> MTFTVDITPKTPTGVIDETKQFTATPSGQTGGGT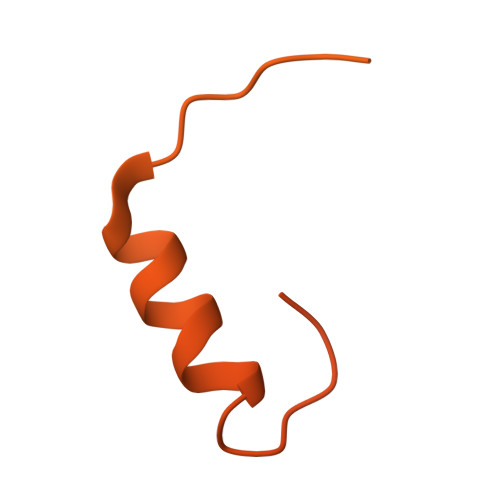ITYAWSVDNVPQDGAEATFSYVLKGPAGQKTIKVVATNTLSEGGPETAEATTTITVKNKTQTTTLAVTPASPAAGVIGTPVQFTAALASQPDGASATYQWYVDDSQVGGETNSTFSYTPTTSGVKRIKCVAQVTATDYDALSVTSNEVSLTVNKKTMNPQVTLTPPSINVQQDASATFTANVTGAPEEAQITYSWKKDSSPVEGSTNVYTVDTSSVGSQTIEVTATVTAADYNPVTVTKTGNVTVTAKVAPEPEGELPYVHPLPHRSSAYIWCGWWVMDEIQKMTEEGKDWKTDDPDSKYYLHRYTLQKMMKDYPEVDVQESRNGYIIHKTALETGIIYTYP(2S)-2-(naphthalen-1-yloxy)-N-[2-(pyridin-4-yl)-1,3-benzoxazol-5-yl]propanamide 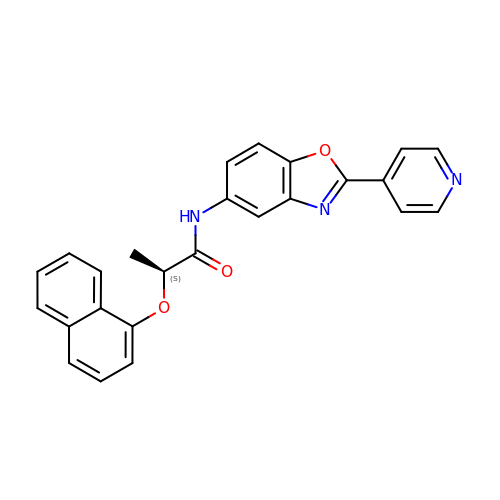| C25 H19 N3 O3 | QCNXGTHMVPSAAC-INIZCTEOSA-N> GSHMGDFVVVYTDGCCSSNGRRRPRAGIGVYWGPGHPLNVGIRLPGRQTNQRAEIHAACKAIEQAKTQNINKLVLYTNSMFTINGITNWVQGWKKNGWKTSAGKE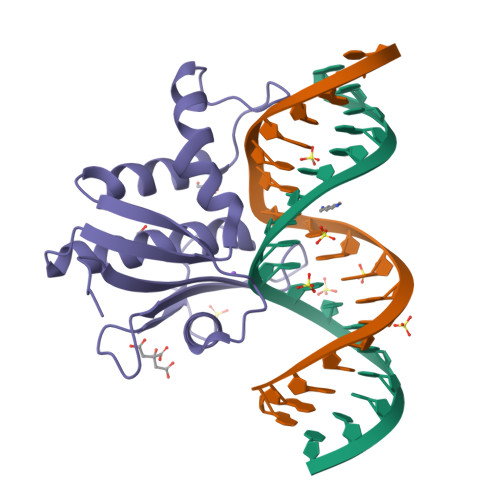VINKEDFVALERLTQGMDIQWMHVPGHSGFIGNEEADRLAREGAKQSED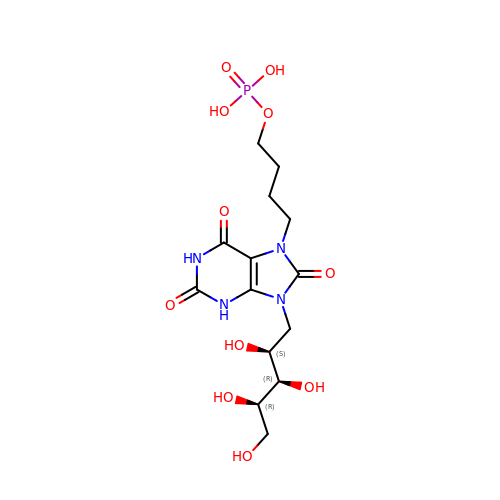4-{2,6,8-TRIOXO-9-[(2S,3R,4R)-2,3,4,5-TETRAHYDROXYPENTYL]-1,2,3,6,8,9-HEXAHYDRO-7H-PURIN-7-YL}BUTYL DIHYDROGEN PHOSPHATE | C14 H23 N4 O11 P | VBXZSBKAJFXURR-QXFUBDJGSA-N> MKRIFRSSVRVGAALPLGAVVPAIFYCNGIRIMGRQYTHDTYRPFGDGYKEVRGTAPTDECNLLFASLNDESLPLCEDSGNVVNGQLVRASALVDSDALADSQELVDVAIEEDRREEEDNSVLLVPXHEEQNSVTKKQNEGEDVTTRCDHLFSVVGCPTTVSTATSGIPNTPSRNYLSEQDALYLSPTTPEEARVPSALCPQLSACVMVVFAANDMRVHDNYALALAATRAEAAGGLPVIAVTVVDYRMFAQPSAVGGFFRQSPMRARFFLETLAALRYKLERELRIPLLVRCGRPEDHIPRLVVEC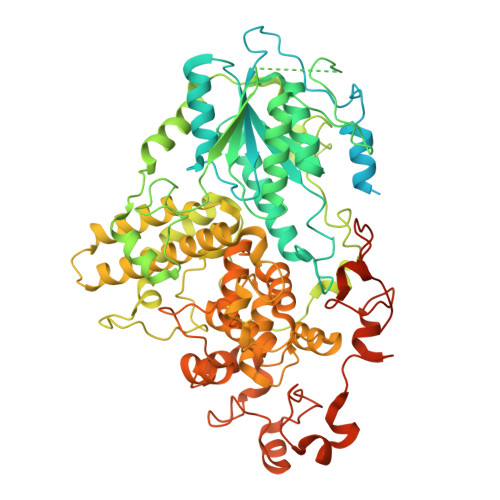GAIDVFLTTQYAPHEKEVHNDIVEAINQRRWVSRDPTAGYKAIEHDATVVHPFGATSASTKVGVKESRLTAAPVAHSVWQTTLVHIDDLPVPVASMVEGERWYHDDVTTANIRPTAAFDRCINRLSDLPARGDLLPTTGELSGLEPPPLYRGRAPTLVELGYGSPEAFIEEEVIATQSSHPPGEDAAIERVLDWLMDGGMTSMLRYGRDRRTNTKMYSQRLSRLSPYLSCGALSPRRFYEELRRFTSEHLRDNFVQQQYREALLRLSRRDYWHWMGLRYGPLLFYEYGPRPEHTDDIADWRHDPKIVQKWCAGLTGIPFADAAMRELTLTGFVADEGRQGLIWLLSRGYGQDWRLGAEWLERCSIDYDPFVCYGNCAYYSELVRDDFGETVRNIHWLAHHHDQTGIYVKKWLPQLSKIPPVYIHRPHVLTERMQAMHGVQLGKNYPYPLKLWDGAQYTLSSEHLTTYFSEGSQWHRKAKNGAGGSGYAEALRHGTVILEPHQLQSSAFGELEHGVMHTVPVVKDDTAGRGQHNRSLTASDE> GALPDPVKPKAPKAVNPFHLGMAGYTFVNFDLDTTLKTLERLDIHYLCIKDFHLPLNSTDEQIRAFHDKCAAHKVTGYAVGPIYMK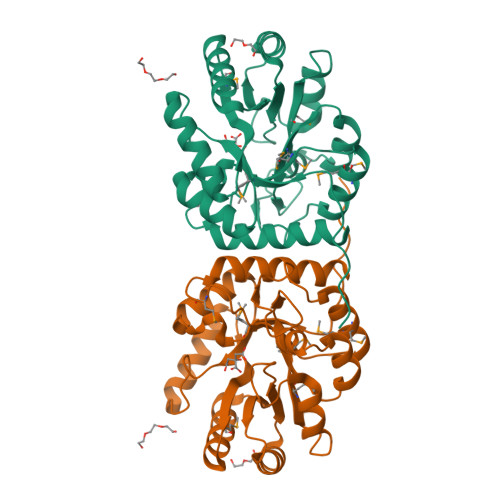SEEEIDRAFDYAKRVGVKLIVGVPNYELLPYVDKKVKEYDFHYAIHLHGPDIKTYPDATDVWVHTKDLDPRIGMCLDVGHDLRNGCDPVADLKKYHTRVFDMHIKDVTDSSKAGVGIEIGRGKIDFPALIRMMREVNYTGMCSLEYEKDMKDPFLGIAESIGYFKAVSDLT>[2x]SMHEYDVGKLKVEHPWLRAPADGEKNASFYAFIHNNGDTPDKLVAVKVEKFGSAVIHGDAKNLALEAP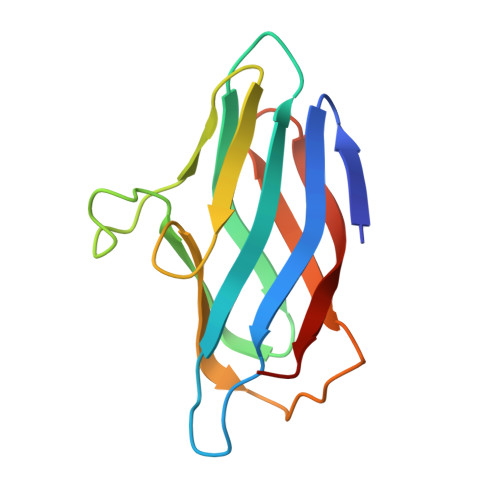VLLPPKQKITLAPGGAYVALLDAKKHLEVGWGLEMTLVFEKAGEVVIDAAIDAPD>TVTYTNRVADARLGTFSQLLLQWKGSIYKLLYSEFLIFISLYFAISLVYRLILSESQRLMFEKLALYCNSYAELIPVSFVLGFYVSLVVSRWWAQYESIPWPDRIMNLVSCNVDGEDEYGRLLRRTLMRYSNLCSVLILRSVSTAVYKRFPSMEHVVRAGLMTPEEHKKFESLNSPHNKFWIPCVWFSNLAVKARNEGRIRDSVLLQGILNELNTLRSQCGRLYGYDWISIPLVYTQVVTVAVYSFFLACLIGRQFLDPEKAYPGHELDLFVPVFTFLQFFFYAGFLKVAEQLINPFGEDDDDFETNWLIDRNLQVSLMA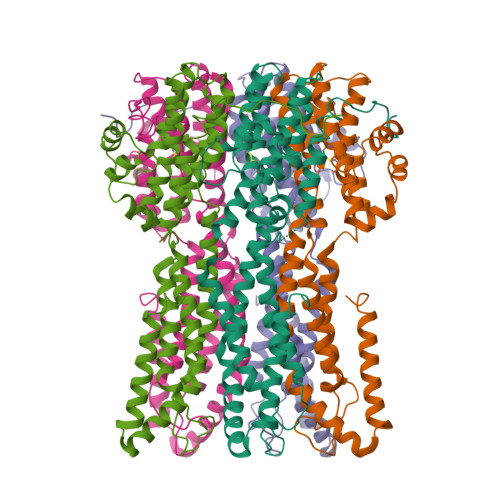VDEMHQDLPILEKDLYWNEPDPQEGEEF[5x]>[2x]SNAMRIGVIMGGVSSEKQVSIMTGNEMIANLDKNKY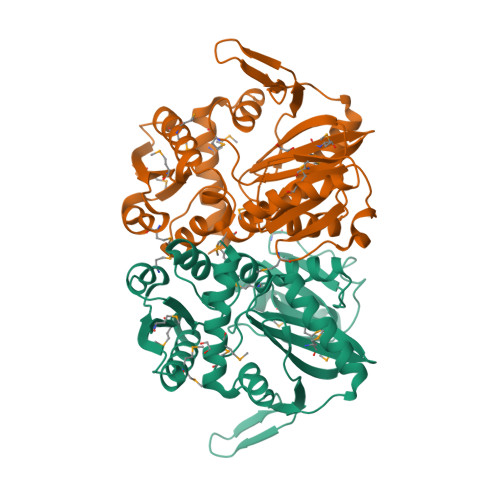EIVPITLNEKMDLIEKAKDIDFALLALHGKYGEDGTVQGTLESLGIPYSGSNMLSSGICMDKNISKKILRYEGIETPDWIELTKMEDLNFDELDKLGFPLVVKPNSGGSSVGVKIVYDKDELISMLETVFEWDSEVVIEKYIKGEEITCSIFDGKQLPIISIRHAAEFFDYNAKYDDASTIEEVIELPAELKERVNKASLACYKALKCSVYARVDMMVKDGIPYVMEVNTLPGMTQASLLPKSADAAGIHYSKLLDMIIETSLRVRKEEGF>XGKIEQILQKIEKILQKIEWILQK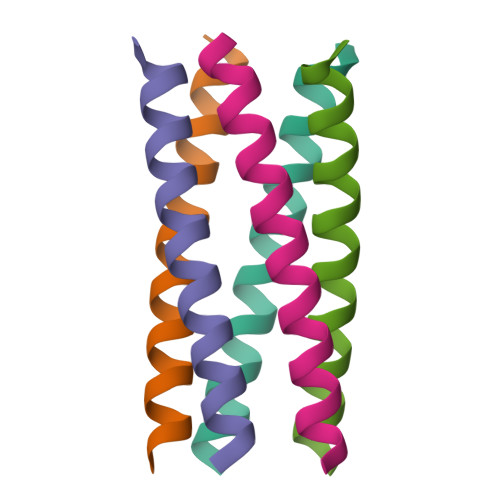IEQILQG[10x]> MEAPVYLCLLGNDPAPAYLGLKVVEREAGRVAKAVFYSFPAWNEEYGKKRQAFFRLLSEKGVLYEERPLEKGLEEAEAREVWVNLTGGAKYWAVRFLGHWRRPGARVFLVEGHRALEAPRALFLWPREEERSLEAEALTLEEYARLYLEPLGEAWERVSPPGAFPPGAQAARLPGREGGVFVVHRGLPYWYWVRPHLGGEAKDMSRKALSAFSGEAKRLGGQLCLPVVPYHKAHLRSRHPKERENVFARWRAWAREYGVFLVDPGRPLEEEVASLIKGKASKKALPLPQEGPLLLALVSEQAVPLYAAYLHAGPREVYLLTTPEMESRLRWAEAFFRGKGVRVHRSFLSGPWALREVRDLLAPVVEEALRRGHPVHANLNSGTTAMALGLYLALRDGARAHYLDGDRLLLLDGGEAEVPWEEGRPEDLLALRGYRFEEEYPDARPDPGLLALAEEILRRWDEVQTSWEASPLVRRFLKFWKKRFGQAFPPKRLSRLKGLPLEYAVYSHLNAHLAPKGGQARMGGHLVPLGGNEALAPQSTEVDGVFFHRGALWFVECKPTDEGLRERAPIMAELVRSVGGVEARGLMVARRWRGAPPPASPNLVYMALEGGEGVGVYRFPEELEKALSRNPAPRRGLE

Type III (Csm/Cmr) CRISPR systems utilise a cyclase domain in the Cas10 subunit to generate cyclic oligoadenylate (cOA) by polymerising ATP1–3. TTHB155, hereafter Can1 (CRISPR ancillary nuclease 1), was identified as a potential accessory protein of the type III CRISPR system by Shah et al. in 2018 (cluster 107). Here, we show that Can1 is a metal dependent DNA nuclease, activated by cA4 binding. Once activated by cA4 generated in response to detection of foreign RNA, Can1 cleaves supercoiled DNA to generate nicked products.

Can1, with selenomethionine incorporated, was crystallised in the presence of cA4. Diffraction data were collected at Diamond Light Source to 1.83 Å resolution and phased using the incorporated selenium atoms. The protein chain is traced from residue 3 to 638, with three short sections too disordered to model (464-471, 491-494 and 530-539). The structure of Can1 is unique, with four distinct domains linked by flexible loops. At the N-terminus there is a CARF domain (residues 3-151), domain 2 (residues 168-276), a second CARF domain (residues 293-422) and a nuclease domain (residues 426-638). The molecule of cA4 sits at the interface between the two CARF domains of Can1 and is completely enclosed by the protein. There are a fairly modest number of hydrogen bond interactions between Can1 and cA4 given its size, all but one of which originate from the two CARF domains. Can1 is unusual in being a monomeric protein with two non-identical CARF domains, and therefore possesses less intrinsic symmetry than most family members. cA4 is bound in a markedly asymmetrical conformation, which is in part exaggerated by the position of one adenine base in an axial position, driven by a stacking interaction with a tryptophan residue. The cA4 ligand is completely buried in the Can1 complex, demonstrating that significant protein conformational changes are required to facilitate binding. Modelling of dsDNA binding by the nuclease domain, coupled with the observation that conserved basic residues in the nuclease-like domain are essential for activity (presumably due to a role in DNA binding rather than directly in catalysis), suggests that cA4 binding allows the nuclease and nuclease-like domains to assemble into a functional dsDNA binding site, activating the enzyme.> TFPIMSNFERDFVIQLV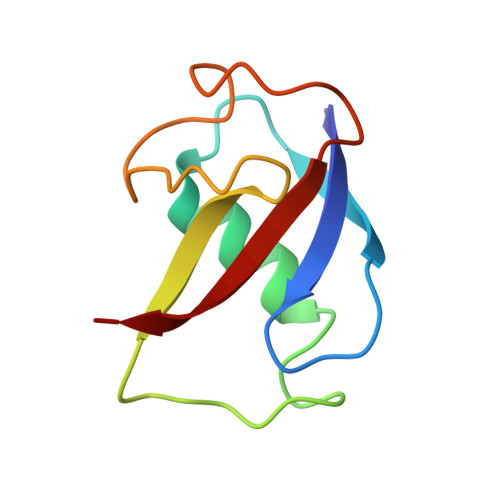PVDTEDTMDQVAEKCAYHSINRRVHPQPEKILRVRRHEDGTLFPRGMIVSDAGLRPTETLDIIFMD>GSHMSLFDFFKNKGSAATATDRLKLILAKERTLNLPYMEEMRKEIIAVIQKYTKSSDIHFKTLDSNQSVETIEVEIILPR[2x]

MinE has two structurally and functionally distinct domains: the anti-MinCD domain and the topological specificity domain (TSD). In contrast, the anti-MinCD domain of EcMinE (residues 1–31) interacts with MinD and induces the dissociation of the MinCD complex, thereby blocking the inhibitory action of MinC on cell division. Here we report the crystal structure of full-length Helicobacter pylori MinE (HpMinE) and redefine the TSD of HpMinE based on that structure. Remarkably, we found that the N-terminal region of the TSD (residues 19–26), which was previously defined as part of the anti-MinCD domain, forms a β-strand (βA) that participates in TSD folding, and HpMinE forms a dimer through the interaction of anti-parallel βA-strands.

The crystal structure of full-length HpMinE was solved using the multi-wavelength anomalous dispersion (MAD) method and refined to an Rwork = 26.2% and Rfree = 29.6% at 2.8 Å resolution. Two monomers were observed in an asymmetric unit; they formed a homodimeric α/β structure with an upper surface (the α-face) consisting of α-helix and a lower surface (the β-face) consisting of an anti-parallel twisted β-sheet. The extensive hydrophobic dimer interface subsumed about 1100 Å2 of surface area (22.8% of the total surface area), and size exclusion chromatography showed that HpMinE forms a stable dimer in solution (data not shown). Each monomer is composed of a long helix αA (residues 35–50) and a three-stranded anti-parallel β-sheet comprised of βA (residues 19–26), βB (residues 54–59) and βC (residues 67–74). The N-terminus of HpMinE (residues 1–12 in MolA; residues 1–15 in MolB) was disordered and invisible within the crystal structure. Within the crystal packing, HpMinE forms the spiral structure with 12 protomers per turn generated by the sixfold symmetry. The formation of the polymeric structure is entirely attributable to the dimer–dimer interaction mediated by the anti-parallel βB-strand. To further analyse the dimer–dimer interaction observed in the crystal structure of native HpMinE, we compared the crystal structures of HpMinE crystallized in two different space groups. Native and Se-Met-labelled crystals of HpMinE were crystallized in the P64 and P65 space groups respectively. The conformation of the dimer was well conserved in the two crystal forms, but the dimer–dimer interaction began to deviate in the tetramer formation, and the packing was tilted about 24° in hexamers.>[2x]MAPPAVLSKSGVIYGKDV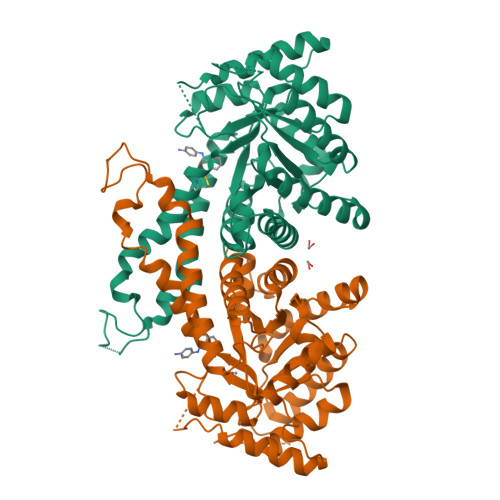KDLFDYAQEKGFAIPAINVTSSSTVVAALEAARDNKAPIILQTSQGGAAYFAGKGVDNKDQAASIAGSIAAAHYIRAIAPTYGIPVVLHTDHCAKKLLPWFDGMLKADEEFFAKTGTPLFSSHMLDLSEETDDENIATSAKYFERMAKMGQWLEMEIGITGGEEDGVNNEHVEKDALYTSPETVFAVYESLHKISPNFSIAAAFGNVHGVYKPGNVQLRPEILGDHQVYAKKQIGTDAKHPLYLVFHGGSGSTQEEFNTAIKNGVVKVNLDTDCQYAYLTGIRDYVTNKIEYLKAPVGNPEGADKPNKKYFDPRVWVREGEKTMSKRIAEALDIFHTKGQLHHHHHH3-(2-amino-1,3-benzothiazol-6-yl)-1-{[2-(4-methylpiperazin-1-yl)quinolin-3-yl]methyl}-1H-pyrazolo[3,4-d]pyrimidin-4-amine 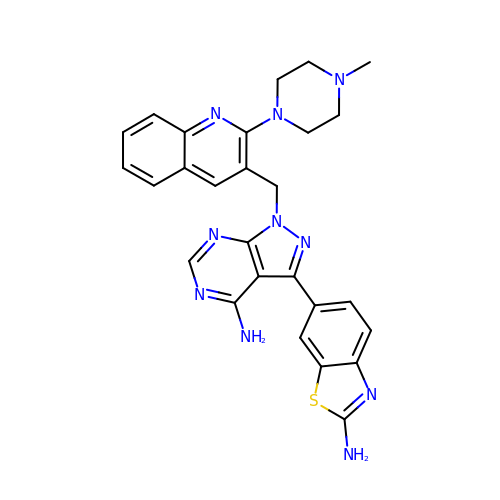| C27 H26 N10 S | UNSGOTITAWKECZ-UHFFFAOYSA-N> SHMQSRELKTVSADCKKEAIEKCAQWVVRDCRPFSAVSGSGFIDMIKFFIKVKAEYGEHVNVEELLPSPITLSRKVTSDAKEKKALIGREIKSAVEKDGASATIDLWTDNYIKRNFLGVTLHYHENNELRDLILGLKSLDFERSTAENIYKKLKAIFSQFNVEDLSSIKFVTDRGANVVKSLANNIRINCSSHLLSNVLENSFEETPELNMPILACKNIVKYFKKANLQHRLRSSLKSECPTRWNSTYTMLRSILDNWESVIQILSEAGETQRIVHINKSIIQTMVNILDGFERIFKELQTCSSPSLCFVVPSILKVKEICSPDVGDVADIAKLKVNIIKNVRIIWEENLSIWHYTAFFFYPPALHMQQEKVAQIKEFCLSKMED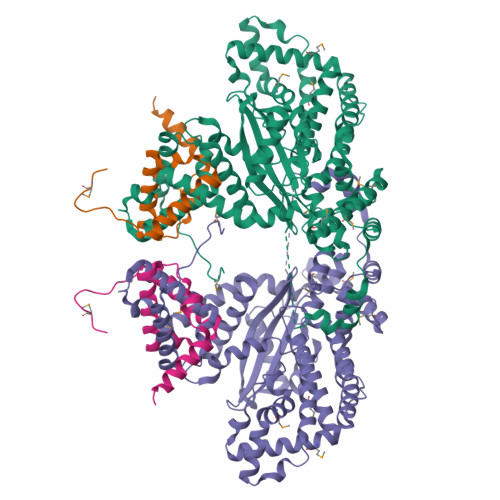LELINRMSSFNELSATQLNQSDSNSHNSIDLTSHSKDISTTSFFFPQLTQNNSREPPVCPSDEFEFYRKEIVILSEDFKVMEWWNLNSKKYPKLSKLALSLLSIPASSAASERTFSLAGNIITEKRNRIGQQTVDSLLFLNSFYKNFCK;> SHMQSRELKTVSADCKKEAIEKCAQWVVRDCRPFSAVSGSGFIDMIKFFIKVGAEYGDHVNVEELLPSPITLSRKVTSDAKEKA>SNAKIGVLQFVSHPSLDLIYKGIQDGLAEEGYKDDQVKIDFMNSEGDQSKVATMSKQLVANGNDLVVGIATPAAQGLASATKDLPVIMAAITDPIGANLVKDLKKPGGNVTGVSDHNPAQQQVELIKALTPNVKTIGALYSSSEDNSKTQVEEFKAYAEKAGLTVETFA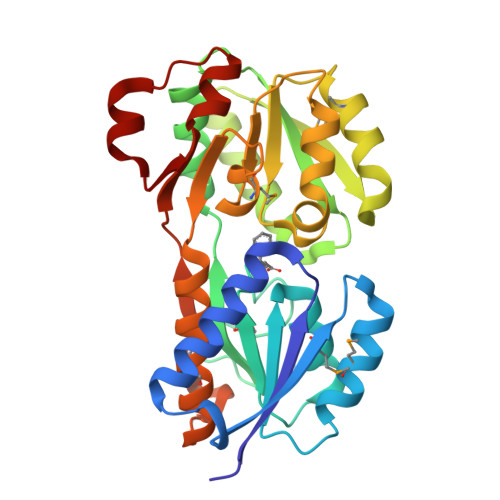VPSTNEIASTVTVMTSKVDAIWVPIDNTIASGFPTVVSSNQSSKKPIYPSATAMVEVGGLASVVIDQHDLGVATGKMIVQVLKGAKPADTPVNVFSTGKSVINKKIAQELGITIPESVLKEAGQVI[2x]> MSDNDELQQIAHLRREYTKGGLRRRDLPADPLTLFERWLSQACEAKLADPTAMVV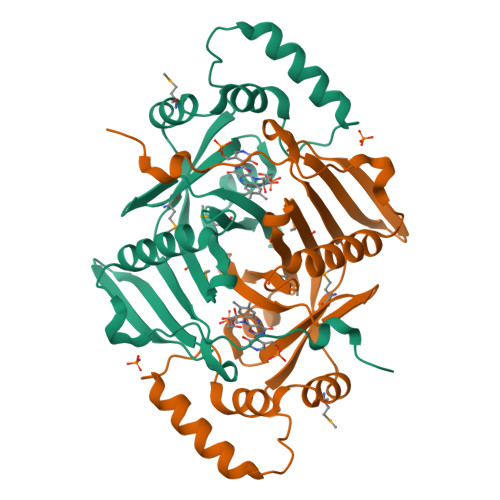ATVDEHGQPYQRIVLLKHYDEKGMVFYTNLGSRKAHQIENNPRVSLLFPWHTLERQVMVIGKAERLSTLEVMKYFHSRPRDSQIGAWVSKQSSRISARGILESKFLELKQKFQQGEVPLPSFWGGFRVSLEQIEFWQGGEHRLHDRFLYQRENDAWKIDRLAP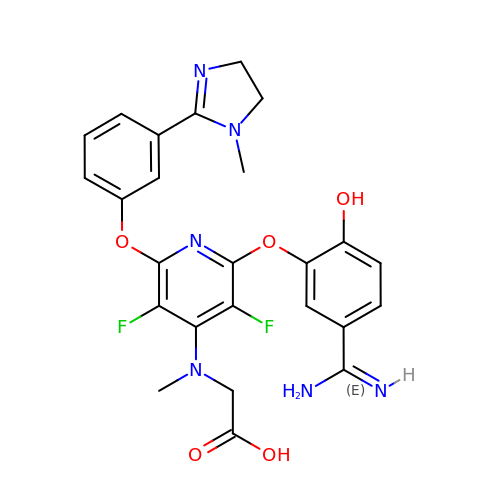N-[2-[5-[AMINO(IMINO)METHYL]-2-HYDROXYPHENOXY]-3,5-DIFLUORO-6-[3-(4,5-DIHYDRO-1-METHYL-1H-IMIDAZOL-2-YL)PHENOXY]PYRIDIN-4-YL]-N-METHYLGLYCINE | C25 H24 F2 N6 O5 | NPNSVNGQJGRSNR-UHFFFAOYSA-N>MAHHHHHHSSGLEVLFQGPMTERLETRPQALLIKVPTEIVVKVVDDVDVAAPAVGQVGKFDDELYDEAGAQIGTSSGNFRIEYVRPTDGGLLTYYQEDITLSDGVIHAEGWADFNDVRTSKWVFYPATGVSGRYLGLTGFRQWRMTGVRKSAEARILLGE[4x]

The second comprises enzymes which function as explicit [4 + 2] cyclases, including the Diels–Alderase AbyU. This biocatalyst generates the spirotetronate skeleton of the antibiotic natural product abyssomicin C in the marine actinomycete Micromonospora maris AB-18-032 (previously Verrucosispora maris AB-18-032). Structural studies of AbyU have revealed that this enzyme possesses a distinctive β-barrel fold, wherein the barrel lumen constitutes the active site of the enzyme. Access to this site is regulated via a flexible capping loop, with catalysis promoted by the conformational constriction of the linear substrate 3.18 This mechanism is consistent with that proposed for the related cyclase PyrI4, which is derived in part from unliganded and product-bound crystal structures of the enzyme.

To establish the mode of substrate binding in AbyU the substrate analogue 13, a non-transformable counterpart of 5 was designed for use in co-crystallisation studies. Recombinant AbyU was subsequently subjected to crystallisation screening in the presence of substrate analogue 13. Resulting crystals underwent X-ray diffraction analysis which yielded a structure of the AbyU-13 complex to 1.95 Å resolution (Fig. 2 and Table S1†). Inspection of the AbyU-13 complex reveals an overall fold comprising a homodimer of two β-barrels consistent with that previously reported for the polypeptide. Four copies of AbyU were observed in the asymmetric unit (AU), comprising one intact dimer (between chains A and C) and two copies (chains B and D) whose dimer partner resides within a neighboring AU. Electron density corresponding to a single molecule of substrate analogue 13 was observed in the active sites of three of the four copies (chains A, B and D), with a single HEPES molecule in the fourth (chain C; Fig. 2 and S1–S3†). The percentage occupancies of 13 differ in each copy of AbyU; 80% in chain A and 70% in chains B and D. The side-chain of 13 exhibits greater conformational heterogeneity than would be possible in substrate analogue 5, and as a consequence deviates from the s-cis configuration implicitly required to enable catalysis to proceed. Superimposition of each of the four copies of AbyU reveals equivalent side chain conformations for all active site residues with the exception of Met126. The side chain of this residue points away from the active site in each of chains A, B and D, but inwards towards the barrel lumen in chain C (Fig. S2†). In chains A, B and D a single hydrogen bond of 2.8 Å (oxygen–oxygen distance) is observed between the enzyme and substrate analogue 13, formed between the lactone carbonyl of 13 and the side chain of Tyr76. The conformation adopted by substrate analogue 13 in our AbyU-13 crystal structure is consistent with the substrate binding mode indicated to be most favourable and reactive in our simulations.>[2x]GLVPRGSHMAKHLFTSESVSEGHPDKIADQISDAVLDAILEQDPKARVACETYVKTGMVLVGGEITTSAWVDIEEITRNTVREIGYVHSDMGFDANSCAVLSAIGKQSPDINQGVDRADPLEQGAGDQGLMFGYATNETDVLMPAPITYAHRLVQRQAEVRKNGTLPWLRPDAKSQVTFQYDDGKIVGIDAVVLST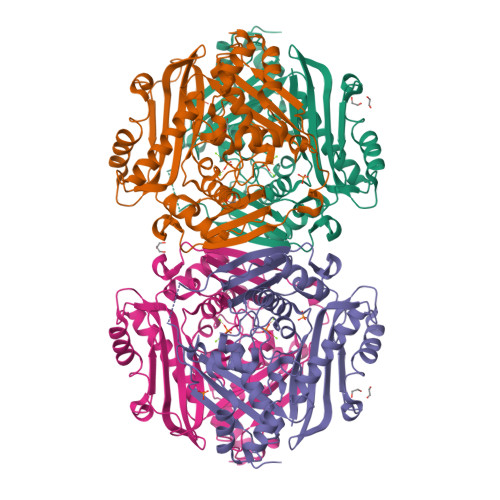QHSEEIDQKSLQEAVMEEIIKPILPAEWLTSATKFFINPTGRFVIGGPMGDCGLTGRKIIVDTYGGMARHGGGAFSGKDPSKVDRSAAYAARYVAKNIVAAGLADRCEIQVSYAIGVAEPTSIMVETFGTEKVPSEQLTLLVREFFDLRPYGLIQMLDLLHPIYKETAAYGHFGREHFPWEKTDKAQLLRDAAGLK>[2x]NNINDSKILSLQNRKNTL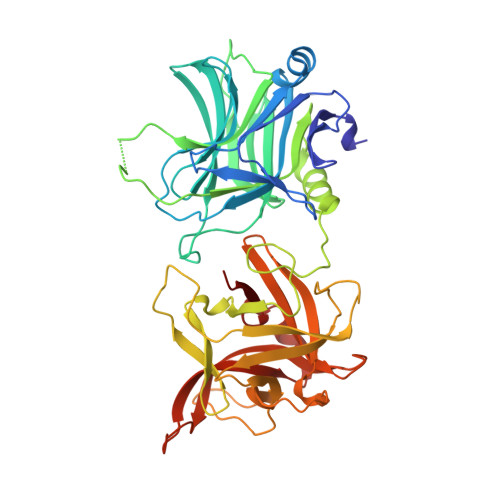VDTSGYNAEVSEEGDVQLNPIFPFDFKLGSSGEDRGKVIVTQNENIVYNSMYESFSISFWIRINKWVSNLPGYTIIDSVKNNSGWSIGIISNFLVFTLKQNEDSEQSINFSYDISNNAPGYNKWFFVTVTNNMMGNMKIYINGKLIDTIKVKELTGINFSKTITFEINKIPDTGLITSDSDNINMWIRDFYIFAKELDGKDINILFNSLQYTNVVKDYWGNDLRYNKEYYMVNIDYLNRYMYANSRQIVFNTRRNNNDFNEGYKIIIKRIRGNTNDTRVRGGDILYFDMTINNKAYNLFMKNETMYADNHSTEDIYAIGLREQTKDINDNIIFQIQPMNNTYYYASQIFKSNFNGENISGICSIGTYRFRLGGDWYRHNYLVPTVKQGNYASLLESTSTHWGFVPVSE The enzyme, pyranose dehydrogenase (PDH), from the filamentous fungus Coprinopsis cinerea (CcPDH) of the Basidiomycete division, is composed of a catalytic PQQ-dependent domain classified as a member of the novel auxiliary activity family 12 (AA12), an AA8 cytochrome b domain, and a family 1 carbohydrate-binding module (CBM1), as defined by the Carbohydrate-Active Enzymes (CAZy) database. In the catalytic cycle of CcPDH, electrons are transferred from the reduced PQQ in the AA12 domain to heme b in the AA8 domain, which acts as a built-in mediator and transfers electrons to a heterogeneous electron acceptor. Therefore, CcPDH is thought to be involved in the extracellular oxidative degradation of the plant cell wall. Here, we present the crystal structures of the AA12 domain in its apo- and holo-forms and the AA8 domain of this enzyme.

The apo-AA12 domain crystal used for the high-resolution data set diffracted to a 1.5-Å resolution, and the final model was refined to R and Rfree values of 10.7% and 13.4%, respectively. Since molecular replacement using the first diffraction data set was not successful, multiple isomorphous replacement (MIR) was used for the initial phase determination of the apo-AA12 domain crystals soaked in the mother liquor containing Pt, Au, or Hg ions. The asymmetric unit of the apo-AA12 domain crystal contains a single AA12 domain (residues 241 to 649 of the full-length CcPDH) with 1 calcium ion, 1 formate ion, 1 sulfate ion, 2 glycerol molecules, and 778 water molecules. A polyethylene glycol molecule is partially modeled as a triethylene glycol moiety located close to Asp601 in the apo-AA12 domain. The structures of the apo- and holo-AA12 domains are almost identical, with the C-α root mean square deviation (RMSD) being equal to 0.77 Å. In the crystallized apo-AA12 domain, the calcium ion-binding site is completely obscured by adjacent molecules in the crystal symmetry; i.e., Arg606 of the symmetry mate interacts with the sulfate ion, which is a calcium ion ligand, via two hydrogen bonds. This crystal packing arrangement appears to prevent PQQ binding, which explains why soaking PQQ to obtain the crystallized holostructure did not succeed. The soaking method was not successful for obtaining the holo-form structure of the PQQ, most likely due to the way in which the apo-form of the crystal was packed. Therefore, the holo-form of the AA12 domain was prepared in solution and crystallized under different conditions.

> TFVSCPGAPQPRYQMNVANGFRVAPVLGGLTMPRGITLDTRGNLLVVERGRGLTGHTLDANGCVTSSKVVIQDTQINHGIDVHPSGRRIIASSGDIAWSWDYDPATMTATNRRTLVTGMNNFYHFTRTVHISRKYPNLFALNVGSDGNIDVPTRQQNSGRAQIRVFDYDQLPQNGVPFVSQYGRVLGYGLRNDVGITEDRAGNIHSIENSLDNAYRMVNGQRRDIHTNNPAEKVYNLGDPSNPRAIFGGYPDCYTVWEPSDFTDSPKQPGDWFTQDNSGQYTDAWCNANAVKPTLLLPPHTAPLDMKFGLGNDTNLYVALHGSWNRQPPQGYKVVVVPGQYSASGEWSPTAPLAQSRTAWSDLLTNRNENQCSGFGNANCFRPVGLVWSADGQNLYVSSDTSGEVFIIKR> MKILLIGMGGTIASVKGENGYEASLSVKEVLDIAGIKDCEDCDFLDLKNVDSTLIQPEDWVDLAETLYKNVKKYDGIIVTHGTDTLAYTSSMISFMLRNPPIPIVFTGSMIPATEENSDAPLNLQTAIKFATSGIRGVYVAFNGKVMLGVRTSKVRTMSRDAFESINYPIIA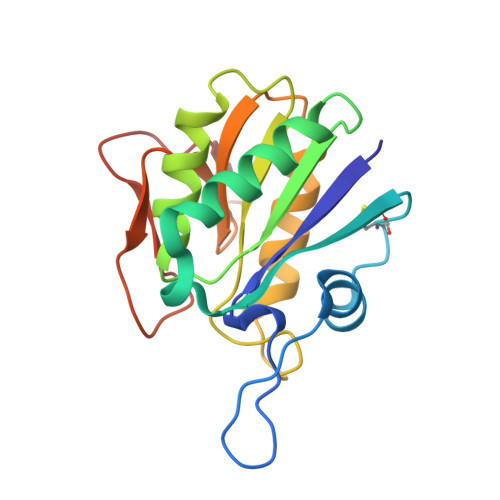ELRGED>[2x]MAEFIYTMKKVRKAHGDKVILDDVTLSFYPGAKIGVVGPNGAGKSSVLRIMAGLDKPNNGDAFLATGATVGILQQEPPLNEDKTVRGNVEEGMGDIKIKLDRFNEVAELMATDYTDELMEEMGRLQEELDHADAWDLDAQLEQAMDALRCPPADEPVTNLSGGERRRVALCKLLLSKPDLLLLDEPTNHLDAESVQWLEQHLASYPGAILAVTHDRYFLD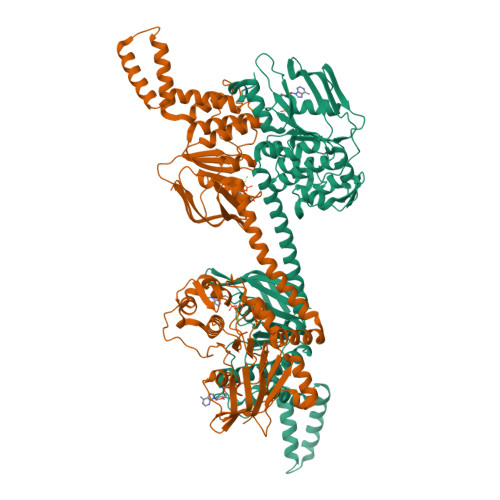NVAEWILELDRGRAYPYEGNYSTYLEKKAERLAVQGRKDAKLQKRLTEELAWVRSGAKARQAKSKARLQRYEEMAAEAEKTRKLDFEEIQIPVGPRLGNVVVEVDHLDKGYDGRALIKDLSFSLPRNGIVGVIGPNGVGKTTLFKTIVGLETPDSGSVKVGETVKLSYVDQARAGIDPRKTVWEVVSDGLDYIQVGQTEVPSRAYVSAFGFKGPDQQKPAGVLSGGERNRLNLALTLKQGGNLILLDEPTNDLDVETLGSLENALLNFPGCAVVISHDRWFLDRTCTHILAWEGDDDNEAKWFWFEGNFGAYEENKVERLGVDAARPHRVTHRKLTRG> ACUCGGAUGAT

Here we describe the crystal structures of a DNA 11-mer that forms eight symmetric ps base pairs. Each oligonucleotide strand forms a ps duplex with a crystallographically equivalent strand, resulting in the first example of a DNA crystal structure that contains four different symmetric homo base pairs. Two of these ps duplexes are coaxially stacked in a head-to-head orientation on equivalent C–C(+) base pairs that is structurally equivalent to the stacking interactions in the DNA i-motif. Remarkably, these two duplexes are effectively locked together as a tetraplex through intercalation of the 5′-most A–A base pairs between adjacent G–G pairs in the opposite duplex.

However, the derivative crystals diffracted to higher resolution and had better overall refinement statistics. For these reasons we have chosen to describe the derivative structure except where noted. C2 and BrU3 are unpaired and their nucleobases are perpendicular to the duplex helical axis where they stack with C2 and BrU3 nucleobases from neighboring duplexes. Interestingly, derivative crystals were grown at neutral pH, suggesting that N3 protonation can occur at non-acidic pHs. A7 makes an additional cross-strand hydrogen bond contact with the BrU8 nucleobase (N6–O4) of the partner strand, while water molecules form bridging hydrogen bonds between N6 and a non-bridging phosophate oxygen of the base pair partner for both A7 and A10 pairs. The BrU8 pairing is through symmetric N3–O4 hydrogen bonding. BrU8 also has shorter (2.86 Å) hydrogen bonding distance than the homopurine interactions (3.03 and 3.45 Å for A7 and G9, respectively). Additionally, C2 was nearly completely disordered in the native crystals. This suggests that BrU3 locally stabilizes the pyrimidine packing interactions that orient adjacent tetraplexes in the crystal lattice. Indeed, BrU3 is involved in halogen–halogen interaction with the bromine of BrU3 from and adjacent tetramer. Additionally, the BrU8 5-bromo position makes a potential halogen bond with a phosphate oxygen from A7.> MGSSHHHHHHSSENLYFQGHKRIYVSYGSPVIDGEVDDIWNNVEWNIPRIYSATTQTNAKFKLMWDDNALYVLAEVYDPVLNSANSTPYQQDSVEIF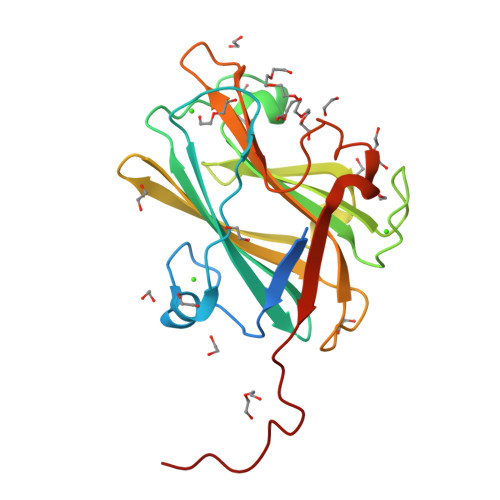LDENFDRAISYQSDDLHYRVNYNNFKTTDAGDILRFYTKTKLLPDGYRVEARIALSKKPINGTIMGFEFQVNEADSSARRVATINMFDNTGNAWQNPSLFGEIKLKGRSDNAVVPINP> MNDQELRAYLSQAKTIAVLGAHKDPSRPAHYVPRYLREQGYRVLPVNPRFQGEELFGEEAVASLLDLKEPVDILDVFRPPSALMDHLPEV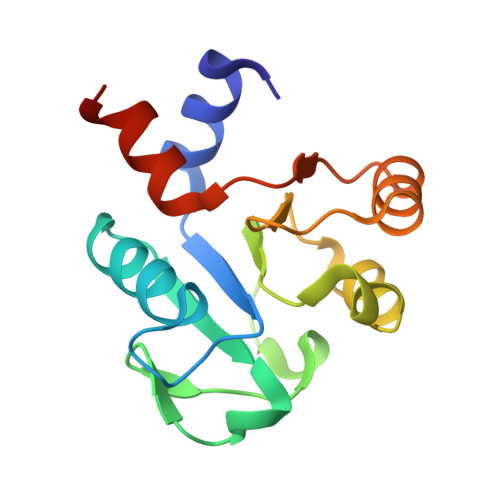LALRPGLVWLQSGIRHPEFEKALKEAGIPVVADRCLMVEHKRLFRGPLPL>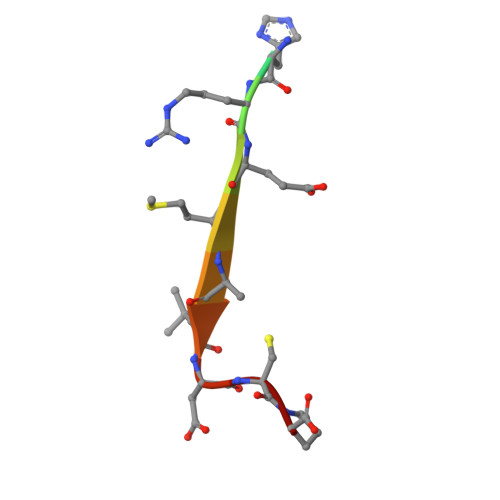 YPKHREMAVDCP>[2x]GPLGSEDDLYRQSLEIISRYLREQATGSKDSKPLGEAGAAGRRALETLRRVGDGVQRNHETAFQGM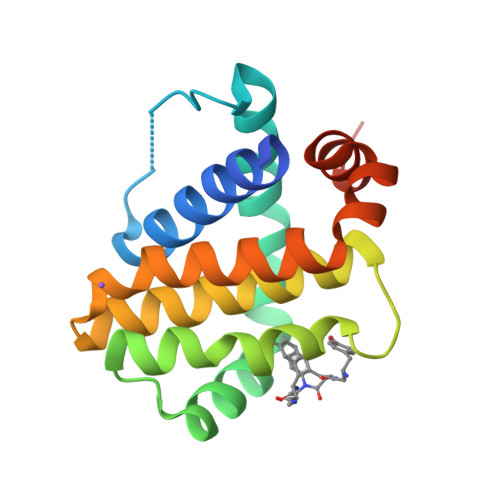LRKLDIKNEDDVKSLSRVMIHVFSDGVTNWGRIVTLISFGAFVAKHLKTINQESCIEPLAESITDVLVRTKRDWLVKQRGWDGFVEFFHVEDLEGG> AIQTRAVINQHGTSETLVENFLGRAALVMMKDF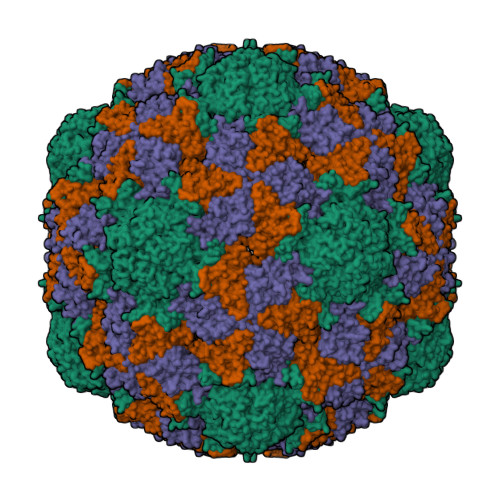EYKNHVTGTQKVQQNFFKWTINTRSYVQLRRKFELFTYIRFDSEITIVPTIRLYTSTGASYSGLPNLTLQAMFVPVGAPTPKSQDSYEWQSACNPSVFFKIDDPPARMTIPFMCINSAYGMFYDGFAGFEKTANGLYGINPANTMGNLCIRVVNAYQPVQYTITIRIYLKPKHIKAWVPRPPRTMPYMSIANTNYTGH;> VLQLKLGNSAIVTQEAANMCCAYGEWPSYLPDNEATAIDKPTQPETSTDRFYTLKSVKWEGTSTGWWWKLPDALNQTGMFGQNVQYHYLYRSGFLCHVQCNATKFHQGALLVVAIPEHQLGKYNTGTSASFDDVMKGKTGGVFTHPYVLDDGTSLACSLIFPHQWINLRTNNSATIMLPWMNCAPMDFALRHNQWTLAIIPVVPLNTSGGTTMVPITVSIAPMCCEFNGLRNAITQ;> GVPTYLLPGSSQFMTTDDHSSAPAFPDFSPTPEIHIPGRVHNMLELVQVESMMEINNVAGSSGMERLRVEISVQTDMDALLFNIPLDIQLDGPLRSTLLANIARYYTHWSGSMEMTFMFCGSFMATGKVILCYTPPGGSCPTDRESAMLGTHIVWDFGLQSSITLVIPWISGSHFRMFNSDAKSINANVGYVTCFMQTNLIVPKEAATSTYIIGFAAAKNDFSLRLMRDSPDI> MGSSHHHHHHSSGLVPRGSHMASADFTQGADVSGNNVTLWFKSSVNTTWVDVHYKVNSGVQQNVRMSFNAGAARFEHTILTAAQAEIEYFFTYNNGVPAYDTTTFTYRSGQPDPEPSTNSIYSIPASSIPQPSEGGVSLKVMNGTGGAYTDDQIYWGVIGINPVNGKWSYLDLAGRLLPISSDLNNAPGHLTKDGINYANIYHKISDANWVNLPKIESGRLFLSVGSPLYMKTFDDGFAGPDLNNPTDPNLNIIFDFVEFTVDKDGYHGNTTRVDQFGFPIQHRLVNLAGNYDRTVGELESETRSGLFAKYVNEVPYEFKSLGTLQAPYRILSPMKGPFQEGGAYENYFAGYSSISTQDILLGVGEASNPEVCAALNRHVYTEPDNWNRVDQYYQAAPANYYAKFWHDHSIDGLAYGFCYDDVNGQAAYLEVGD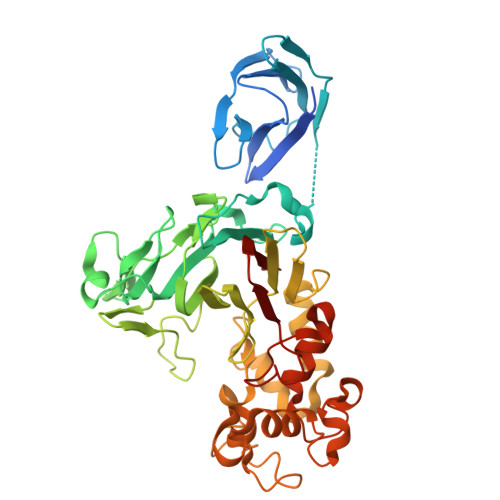PKGLIVRVGW4-AMINO-1-[(1S,3R,4R,7S)-7-HYDROXY-1-(HYDROXYMETHYL)-2,5-DIOXABICYCLO[2.2.1]HEPT-3-YL]-5-METHYLPYRIMIDIN-2(1H)-ONE 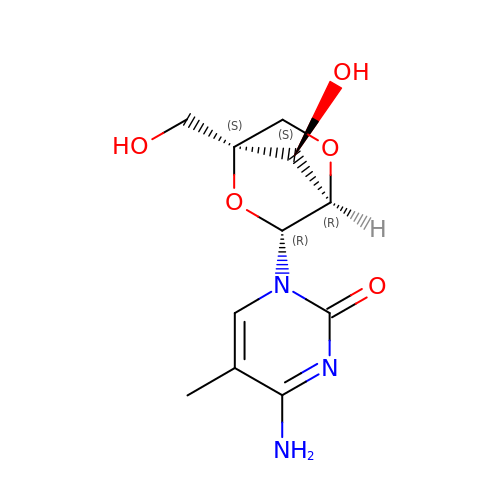| C11 H15 N3 O5 | NELYIRACPIJATH-SZVQBCOZSA-N> MTNATIAPTTTAAPVTKSVDAPTADENTPLFSPSLISPDVL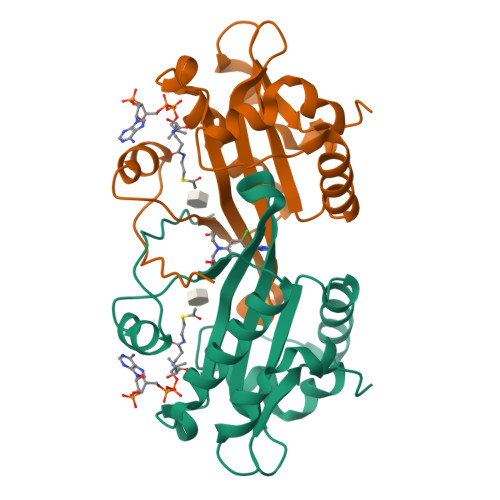AVLPADYTIRPLCRSDYKRGYLDVLRVLTTVGDINEEQWNSRYEWIRARSDEYYLLVVCDGEGRIVGTGSLVVERKFIHSLGMVGHIEDIAVEKGQQGKKLGLRIIQALDYVAEKVGCYKTILDCSEANEGFYIKCGFKRAGLEMAHYY> GSHMEAWFNEKSKELTT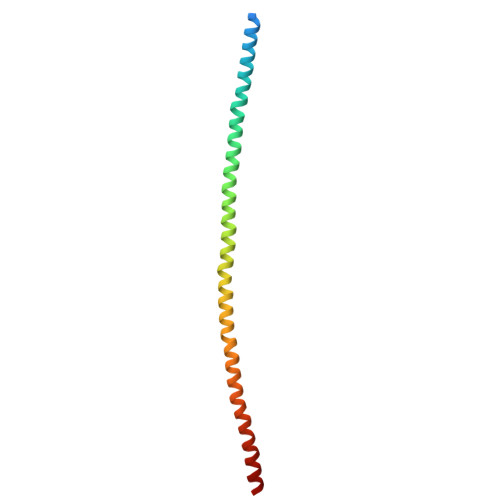EIDNNIEQISSYKSEITELRRNVQALEIELQSQLALKQSLEASLAETEGRYCVQLSQIQAQISALEEQLQQIRAETECQNTEYQQLLDIKIRLENEIQTYRSLLEGE> AMKDHKFWRTQPVKDFDEKVVEEGPIDKPKTPEDISDKPLPLLSSFEWCSIDVDNKKQLEDVFVLLNENYVEDRDAGFRFNYTKEFFNWALKSPGWKKDWHIGVRVKETQKLVA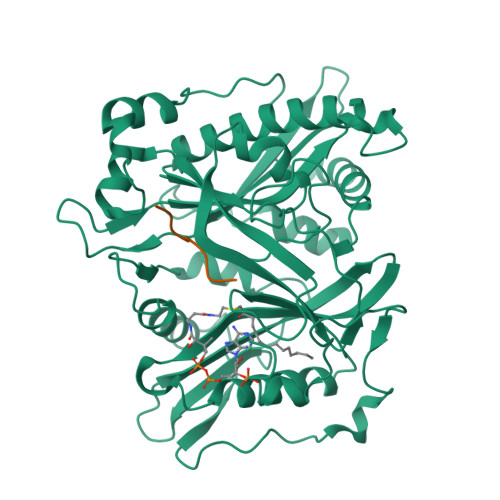FISAIPVTLGVRGKQVPSVEINFLCVHKQLRSKRLTPVLIKEITRRVNKCDIWHALYTAGIVLPAPVSTCRYTHRPLNWKKLYEVDFTGLPDGHTEEDMIAENALPAKTKTAGLRKLKKEDIDQVFELFKRYQSRFELIQIFTKEEFEHNFIGEESLPLDKQVIFSYVVEQPDGKITDFFSFYSLPFTILNNTKYKDLGIGYLYYYATDADFQFKDRFDPKATKALKTRLCELIYDACILAKNANMDVFNALTSQDNTLFLDDLKFGPGDGFLNFYLFNYRAKPITGGLNPDNSNDIKRRSNVGVVML;> GLYASKLA> EDPHLRNRPGKGHNYIDGMTQEDATCKPVTYAGACSSFDVLLEKGKFPLFQSYAHHRTLLEAVHDTIIAKADPPSCDLQSAHGNPCMKEKLVMKTHCPNDYQSAHYLNNDGKMASVKCPPKYELTEDCNFCRQMTGASLKKGSYPLQDLFCQSSEDDGSKLKTKMKGVCEVGVQALKKCDGQLSTAHEVVPFAVFKNSKKVYLDKLDLKTEENLLPDSFV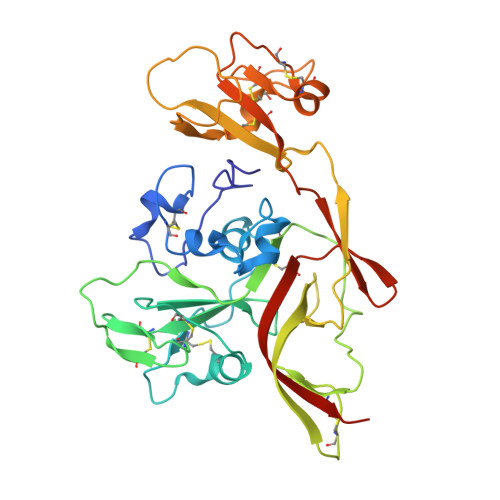CFEHKGQYKGTIDSGQTKRELKSFDISQCPKIGGHGSKKCTGDAAFCSAYECTAQYANAYCSHANGSGIVQIQVSGVWKKPLCVGYERVVVKRELSHHHHHH(4S,5R)-N,N-bis{3-[(2,3-dihydroxybenzoyl)amino]propyl}-2-(2,3-dihydroxyphenyl)-5-methyl-4,5-dihydro-1,3-oxazole-4-carboxamide 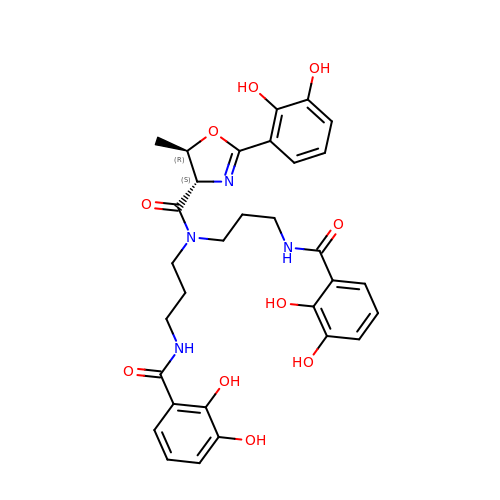| C31 H34 N4 O10 | LHJFXHHBUCCXIF-OSPHWJPCSA-N>NAQKRSPTGIVLMNMGGPSKVEETYDFLYQLFADNDLIPISAKYQKTIAKYIAKFRTPKIEKQYREIGGGSPIRKWSEYQATEVCKILDKTCPETAPHKPYVAFRYAKPLTAETYKQMLKDGVKKAVAFSQYPHFSYSTTGSSINELWRQIKALDSERSISWSVIDRWPTNEGLIKAFSENITKKLQEFPQPVRDKVVLLFSAHSLPMDVVNTGDAYPAEVAATVYNIMQKLKFKNPYRLVWQSQVGPKPWLGAQTAEIAEFLGPKVDGLMFIPIAFTSDHIETLHEIDLGVIGESEYKDKFKRCESLNGNQTFIEGMADLVKSHLQSNQLYSNQLP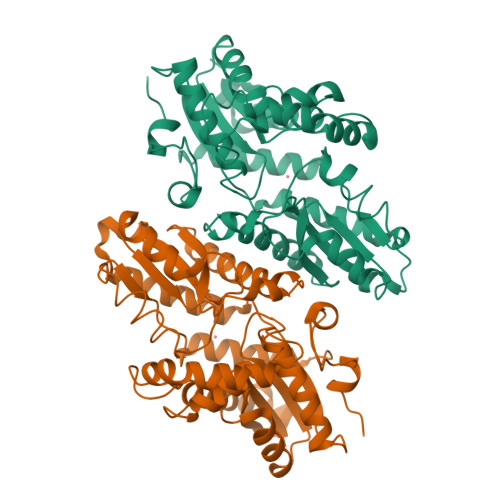LDFALGKSNDPVKDLSLVFGNHEST[2x]farnesyl dihydroxybenzoate | C22 H30 O4 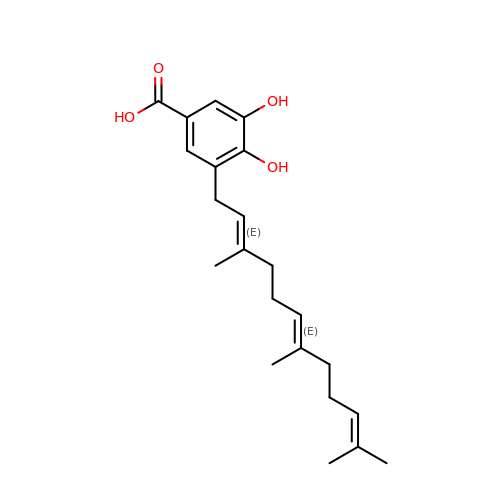| VWHKYMBCXCSQEZ-BTMZFSHUSA-N>[4x]QVVQVNDSMYGFIGTDVVLHCSFANPLPSVKITQVTWQKSTNGSKQNVAIYN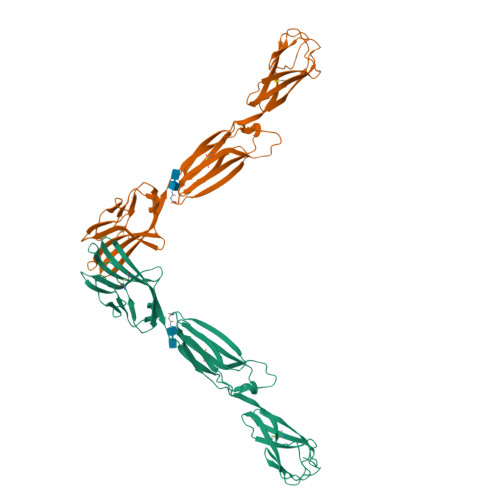PSMGVSVLAPYRERVEFLRPSFTDGTIRLSRLELEDEGVYICEFATFPTGNRESQLNLTVMAKPTNWIEGTQAVLRAKKGQDDKVLVATCTSANGKPPSVVSWETRLKGEAEYQEIRNPNGTVTVISRYRLVPSREAHQQSLACIVNYHMDRFKESLTLNVQYEPEVTIEGFDGNWYLQRMDVKLTCKADANPPATEYHWTTLNGSLPKGVEAQNRTLFFKGPINYSLAGTYICEATNPIGTRSGQVEVNITEFPHHHHHH>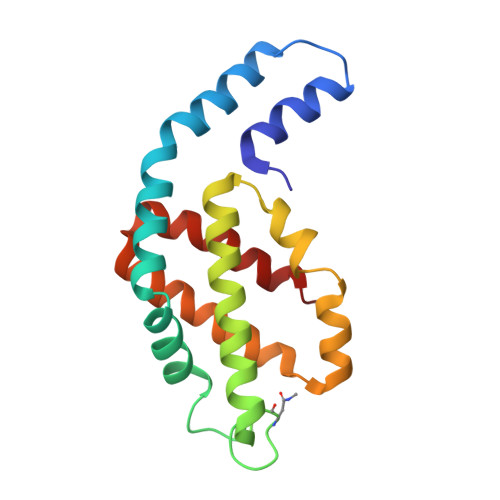 MQDAITAVINASDVQGKYLDTAAMEKLKAYFATGELRVRAASVISANAANIVKEAVAKSLLYSDITRPGGNMYTTRRYAACIRDLDYYLRYATYAMLAGDPSILDERVLNGLKETYNSLGVPIAATVQAIQAMKEVTASLVGADAGKEMGIYFDYICSGLS> MSLGDEIVTRIARVGARHAVHVSPPQGSPGPAAAREGDPIKHASFLGALAGAITGALIGAAVFAAASALVGLTILTGGLATVAVIALGTAATFALGDVISAASSAVTNMVDSIGPPSGTLTSGSPNVFIEGQPAARATTDIAVCSKHPAPPLIAQGSETVLINGSPAARVDDKLACGATIKSGAKTVFIGSGQGTYLAVADEFSAWERAILIAVEFLVPPSRGALKGLGKLFTKPGQGIQGVLKGAKAGAKKAKALLSNRISCAKKAFRETEGAKRYREATKKFFTGDPIDVTTGQLFDQRTDITLGQTLPLVFLRSWVPEEQGLLGPGWTDSFSECALATGDRVEIRTTEGASLYFALPAAYTHSVNPDHPDFTLSRGEQGYILRHRDSPVSKYFTLPHPSSASKEAPRRWLLTEHRDVYDNRLRFIYNKHCQLTQVLHSDGPELTLLYNLRGQLTEIRRTDERLQEVMARYHYHDNGRLAEADSTQNFH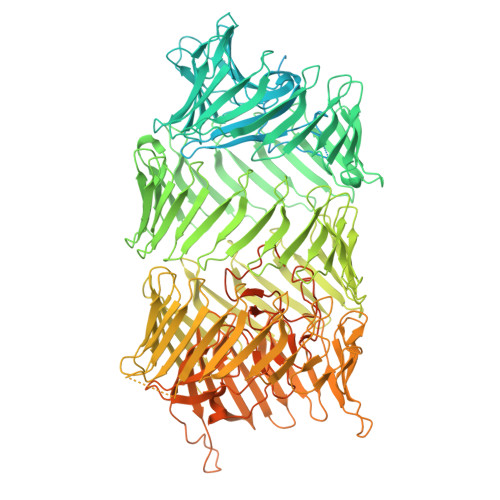LYYEYNAQGLISRWSDGDQTWVDYRYDKQGRCTDSVGAGGFYPVHLDYAPGITRSTTPQGHTTTGHYNDQQLITEIHTPCGGVTRYEYDRWGNLVRQILPEGETLTLTYLADTGRVTSLTEATGAVWQYSYEADSLQLTGMTDPLQRTWLPQYDEQGQPAGFIAPDGRKTTLTRNAFGLVTSETDPDGNSRTQEYDKHQRLVRVLDEENRTVSLGYDSQDRLRSLTAAGALWRWRYDRHHRVAVSDRPDNQLEHFTHDRHGNLTCWTDARGVKWQVEYGPFDLPVARRDGEGHRWQYRYDADTLQLTQVINPQGETYSYTLDADGRVITEQDYAGTQWHYRYDRSGNCIEKRDGEENVTRYDYDAARRLTTLHTPEGPTRYHYDSVGRLLTVDSPDSTLHFEYDGQDRIVREIQPHGEIQRHYPDNRTAERQLLTGETAPVTGPARFSGQTHPGRWQSRREVNRVGELITLTLAGQAPLTIERDDAGRDTGRYVDGGFILRQQYSLMGQLTAQRAGRNPYFFRPAEPDEIEGPAYAGVARRYEYDTALNLTAASDDGQQVNYLLNGNGQVISVGEGRTLREHYQYDETGYPSRRFDGVQEIMGETLYQEGHRLNWVGSHRFVYDRAGRMQEKQFLAEGCRLALTKYRWNSQNQLTGLITPDGIPWEYRYDAFGRRTEKRCIQSGKLTTYLWDGNVPAEIREYQHGRLKMIRHLVFDGWELVAQQTQAFTLNLDNRVELMAGEVQTQYAVSAPTGEPLALFDPAGKRVWRRPKQSLYGLRLGGYGENPQLDPGLRFAGQLFDEESGLFYNRFRYYLPEATCYLSPDPTGLWGGENTYRYVQNPTKFINPLGLAGENVFIHATNKAGFDGIMKSGVLHPNVSGKVAITDVLMSPKDVMRDLLINNPNHIGRGDYAIIFKIDPGERGNIRSPSRLEYTHEGKLKLNNILYAGKNPYAILEHLDYDTRLKLTDNQVKIRKCGGKVDDYKDDDDK The final step in the pathway is catalyzed by a 2-epimerase, which utilizes UDP-2,3-diacetamido-2,3-dideoxy-d-glucuronic acid as its substrate. The focus of this investigation is on the ORF WP_011172736, which we demonstrate encodes for a 2-epimerase. We have also demonstrated that the T. thermophilus enzyme is allosterically regulated by UDP-GlcNAc. Whereas the sugar 2-epimerases that function on UDP-GlcNAc have been the focus of past biochemical and structural analyses, this is the first detailed investigation of a 2-epimerase that specifically utilizes UDP-2,3-diacetamido-2,3-dideoxy-d-glucuronic acid as its substrate.

To determine whether the pH of the crystallization experiments was a contributing factor toward the binding of additional ligands, the next structure (Structure 5) was determined at pH 9.0. Again, the crystals obtained were grown in the presence UDP-GlcNAc3NAcA but in the absence of additional ligands. The model was refined to an overall R-factor of 20.4% at 2.3 Å resolution. Both subunits contained UDP-GlcNAc3NAcA in their active sites. In subunit A, the auxiliary binding pocket was empty whereas in subunit B, electron density corresponding to UDP was observed. The α-carbons for the dimer models determined at either pH 7.0 or pH 9.0 superimpose with an RMSD of 0.2 Å.

>MWVKILSVVGARPQFIKAAAVSRVLRASPGVREVLVHTGQHYDDNMSQVFFEELEIPDPDYHLGIGGGTHGQNTGRMLEAIEGVLLKEKPDWVLVYGNTDSTLAGALAAVKLHIPVAHVEAGLRSFNRRMPEEINRILTDHASDLLFAPTETAVQNLLREGIPENRIHLVGDVMYDAALHYGAKAERKSRILERLGLQAKGYVLATIHRAENTDDQERLRVILEALAEVHQEVPVVFPVHPRTRKRAEAFGLGSYLEKVVALEPVGYLDMVMLEKNARLIVTDSGGVQKEAYFYRVPCVTVREETEWVELLKAEWNYLAAPQNAKDLALTILHRMRTKGVEIDLYGDGRASQKISDFLRKVGIRTLEHHHHHH[2x]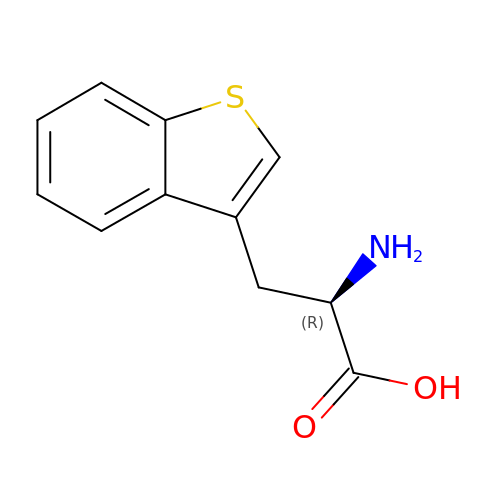(2R)-2-azanyl-3-(1-benzothiophen-3-yl)propanoic acid | C11 H11 N O2 S | GAUUPDQWKHTCAX-SECBINFHSA-N4,4,4-tris(fluoranyl)-1-[4-(4-fluorophenyl)piperidin-1-yl]butan-1-one | C15 H17 F4 N O | 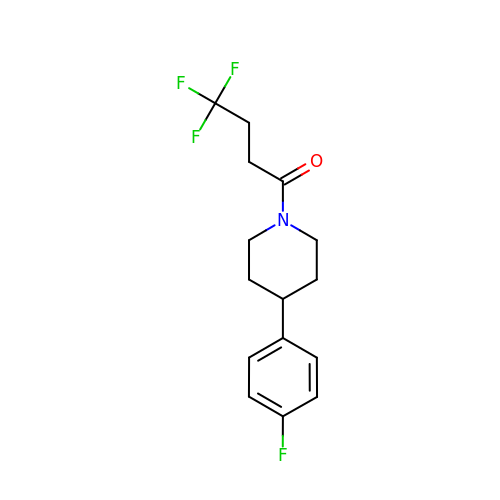ITAKDOUYMNISSA-UHFFFAOYSA-N> XDPADRWCELAAWTCDT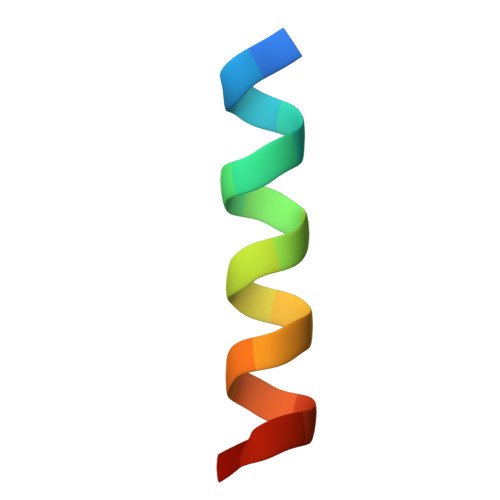FX>AELHLESRGGSGTQLRDGAKVATGRIICREAHTGFHVWMNERQVDGRAERYVVQSKDGRHELRVRTGGDGWSPVKGEGGKGVSRPGQEEQVFFDVMADGNQDI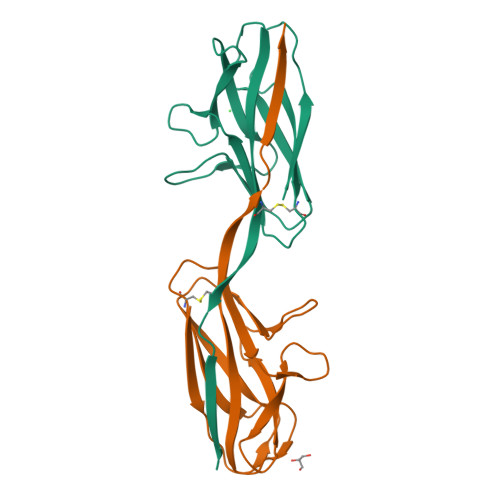APGEYRFSVGGACVVPQEKLAAALEHHHHHH[2x]>MSLSERLKEVQDAVETAMAAAIGRLPAGDLRDAMAYAAQGGKRLRAFLAIESAAIHGISMAQAMPAALAVEALHAYSLVHDDMPCMDNDDLRRGLPTVHKKWDDATAVLAGDALQTLAFELCTDPVLGSAENRVALVAALAQASGAEGMVYGQALDIAAETAAVPLTLDEIIRLQAGKTGALISFAAQAGAILAGADRGPLTAYATALGLAFQIADDILDVEGNEEAAGKRLGKDAEAHKATFVSLLGLAGAKSRAADLVAEAEAALAPYGEAASTLRACA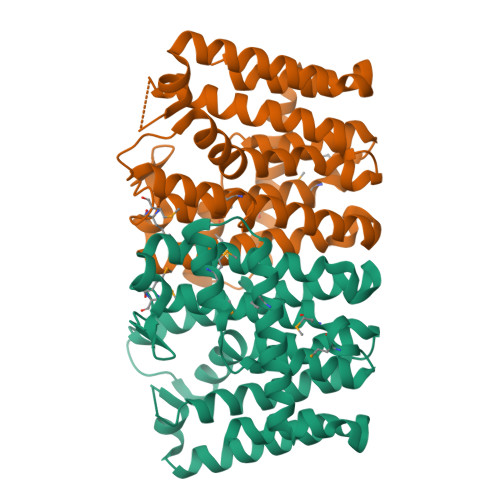RYVIERDKEGHHHHHH[2x]> LTIGNSTITTQEAANIIVGYGEWPSYCSDSDA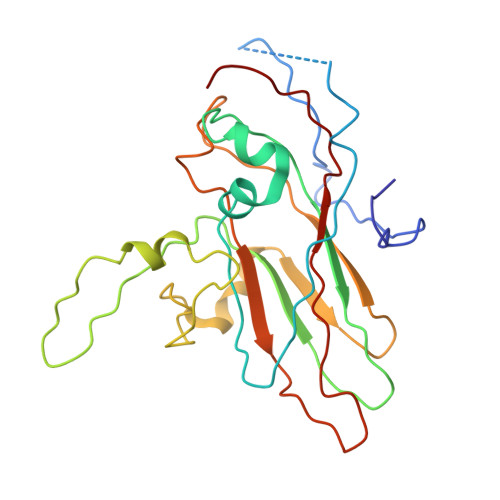TAVDKPTRPDVSVNRFYTLDTKLWEKSSKGWYWKFPDVLTETGVFGQNAQFHYLYRSGFCIHVQCNASKFHQGALLVAVLPEYVIGTVAGGTGTEDSHPPYKQTQPGADGFELQHPYVLDAGIPISQLTVCPHQWINLRTNNCATIIVPYINALPFDSALNHCNFGLLVVPISPLDYDQGATPVIPITITLAPMCSEFAGLRQ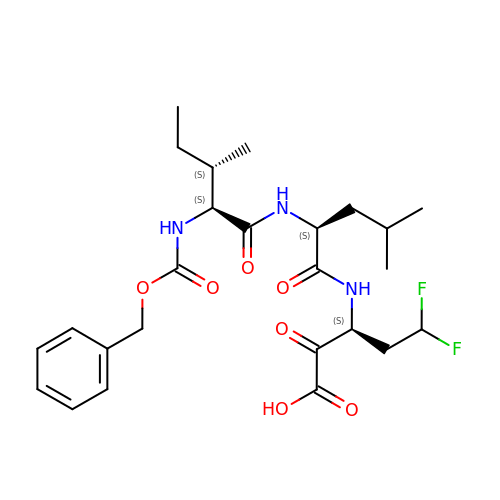N-[(benzyloxy)carbonyl]-L-isoleucyl-N-[(1R)-1-(carboxycarbonyl)-3,3-difluoropropyl]-L-leucinamide | C25 H35 F2 N3 O7 | IXLOEMUNKMDCDV-CAIZAGQASA-N Protein splicing is catalyzed by intervening protein sequences termed inteins. The protein-splicing reaction involves the self-removal of the intein and concomitant joining of the two flanking sequences (exteins). All splicing domains found among inteins have the same structural architecture named HINT (Hedgehog/INTein) which relates to the C-terminal domain of the Hedgehog protein (Hh–C or hog domain). Instead of the N-terminal serine or cysteine missing among class 3 inteins, class 3 inteins contain an additional nucleophilic cysteine residue in block F.

We assumed that introducing the unique WCT motif found in class 3 inteins into a class 1 intein together with the first Cys/Ser to Ala mutation could possibly result in a functional cis-splicing intein if they were closely related by a divergently evolved lineage, similar to class 2 and BIL domains. We introduced the WCT motif on the gp41-1 intein based on the amino-acid sequence alignment. However, the engineered class 3 gp41-1 intein (gp41-1_WCT) produced dominantly the C-cleaved product and only a minute amount of the possible splicing product. To better understand the structural basis for non-productive splicing of the engineered class 3 intein, we solved the crystal structure of gp41-1_WCT at 1.85 Å resolution. Unlike in the crystal structures of MchDnaB1_HAA and MchDnaB1_HN, we observed electron density for the N-terminal extein, confirming that gp41-1_WCT is inactive in proteolytic cleavage at the N-terminal junction (N-cleavage). The catalytic triad of Cys124-His65-Thr143 and Trp67 from the WCT motif in the MchDnaB1 intein can be precisely superimposed with the engineered triad of Cys107-His63-Thr123 and Trp65 (0.39 Å for the r.m.s.d. was obtained for the 35 heavy atoms of these four residues excluding Sγ of Cys124), except for the χ1 angle of the nucleophilic Cys107. The presence of the N-extein (see below) likely induced the trans conformation of Cys107 in gp41-1_WCT. Among the three inteins used in the MD simulations, gp41-1_WCT with the N-extein showed the most abundant population for gauche- and the χ1 angle of the introduced Cys107 was much closer to the ideal 180°-trans conformation than to ~200–210° observed in the other simulations for the two MchDnaB1 inteins. The WCT motif engineering on a class 1 intein did not lead to similar rotational dynamics of the active site residues, indicating that additional compensatory mutations are necessary for splicing-active class 3 inteins. A comparison between the splicing active MchDnaB1 intein and the WCT motif-engineered non-splicing gp41-1 intein derived from a class 1 intein implies that accumulation of random mutations in a class 1 intein would not directly lead to a class 3 intein.

> SGGALDLKTQVQTPQGMKEISNIQVGDLVLSNTGYNEVLNVFPKSKKKSYKITLEDGKEIICSEEHLWPTQTGEMNISGGLKEGMCLYVKEMMLKKILKIEELDERELICIEVSGNHLFYANDILTHN> MEQYYMVIDVAKCQDCNNCFMGCMDEHELNEWPGYTASMQRGHRWMNIERRERGTYPRNDINYRPTPCMHCENAPCVAKGNGAVYQREDGIVLIDPEKAKGKKELLDTCPYGVMYWNEEENVAQKCTMCAHLLDDESWAPK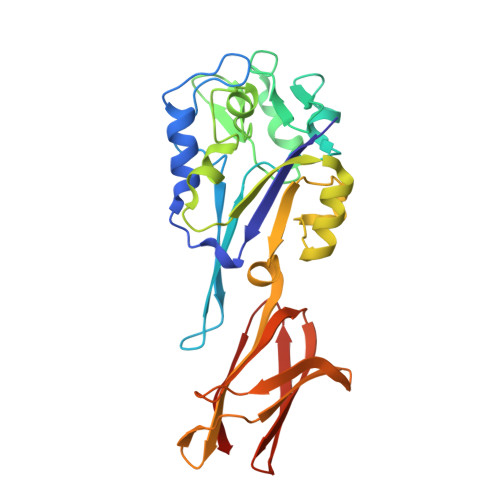MPRCAHNCGSFVYEFLKTTPEAMAKKVEEEGLEVIKPELGTKPRVYYKNLYRFEKNYVTAGILVQGDCFEGAKVVLKSGGKEVASAETNFFGEFKFDALDNGEYTVEIDADGKSYSDTVVIDDKSVDLGFIKL>[2x]MIEPVLENVQPNSAASKAGLQ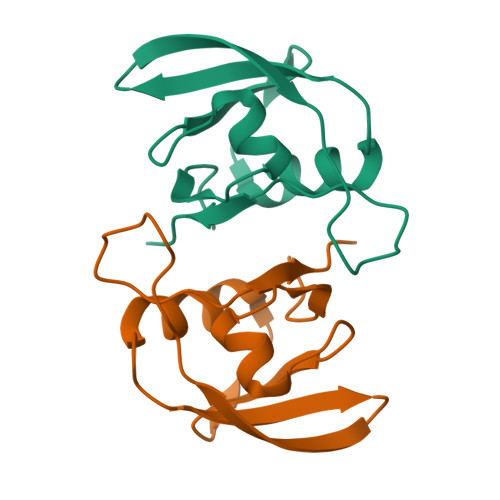AGDRIVKVDGQPLTQWVTFVMLVRDNPGKSLALEIERQGSPLSLTLIPESKPGNGKAIGFVGAEPKVI> GNPFEGVQLWANNYYRSEVHTLAIPQITDPALRAAASAVAEVPSFQWLDRNVTVDTLLVQTLSEIREANQAGANPQYAAQIVVYDLPDRDCAAAASNGEWAIANNGVNNYKAYINRIREILISFSDVRTILVIEPDSLANMVTNMNVPKCSGAASTYRELTIYALKQLDLPHV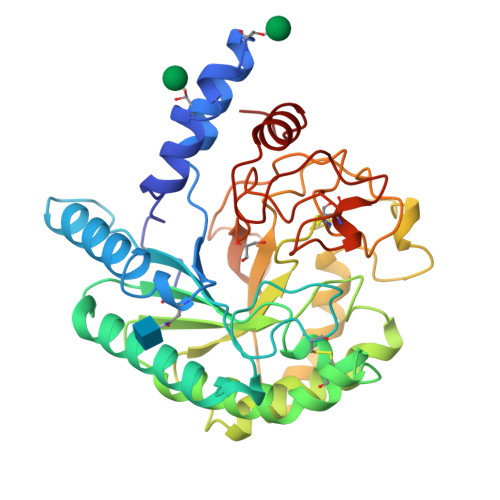AMYMDAGHAGWLGWPANIQPAAELFAKIYEDAGKPRAVRGLATNVANYNAWSVSSPPPYTSPNPNYDEKHYIEAFRPLLEARGFPAQFIVDQGRSGKQPTGQKEWGHWCNAIGTGFGMRPTANTGHQYVDAFVWVKPGGECDGTSDTTAARYDYHCGLEDALKPAPEAGQWFNEYFIQLLRNANPPF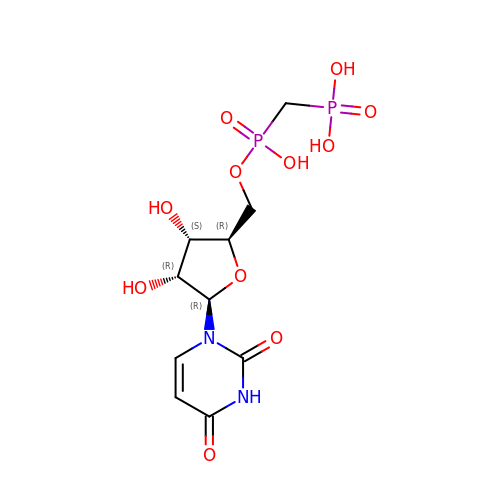5'-O-[(S)-HYDROXY(PHOSPHONOMETHYL)PHOSPHORYL]URIDINE | C10 H16 N2 O11 P2 | PDEGDTTUBZXACY-ZOQUXTDFSA-N> GPLGSMASEERTSALRIRCAHCDAVFDERALPYDADVDSLASSALREKFVRLSLDSESVEFLNRARARGRDECERLARKCTELRRTMSLTEANAILGRGKMFVFSDAHVETLMRACGEGAGGGWFLDVGAGEGEVTRTLARRFAGTCATESSP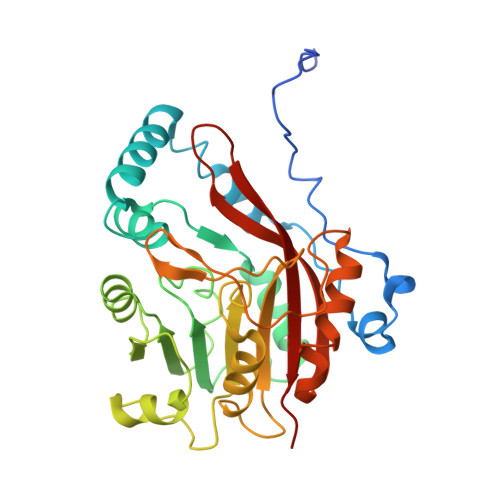GMASRLREKGFDVVLESDTVENVVRETRARGGDVSEDGFDVVAALNLCDRVRSPRALLRDLKRALKAKTGILILAIVVPFRPFVENADGTRSQPDERLDVPSAGSWESGVDALWTELIAPLGFDLVTLSRVPYISEGDHLYDAYVLDDAVFVLRAPP>[8x]MAHHHHHHMKQRTLSIIKPDALKKKVVGKIIDRFESNGLEVIAMKRLHLSVKDAENFYAIHRERPFFKDLIEFMVSGPVVVMVLEGKDAVAKNRDLMGATDPKLAQK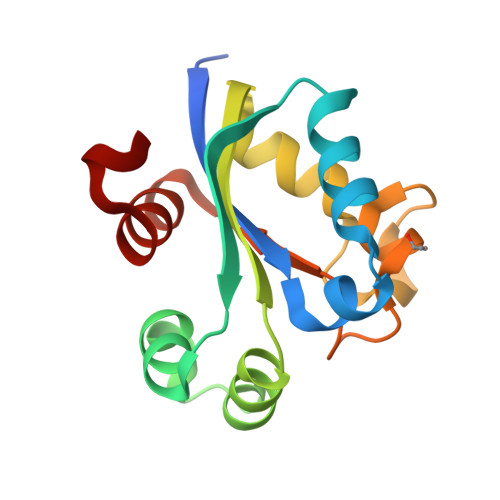GTIRADFAESIDANAVHGSDSLENAHNEIAFFFAARDL> IPCGESCVWIPCISSAIGCSCKSKVCYRNG;> IPCGESCVWLPCISSAIGCSCKSKVCYRNG

Cyclotides are a large family of topologically unique peptides characterized by a head-to-tail cyclic backbone and three interlocked disulfide bonds. This combination of structural features forms a cyclic cystine knot (CCK) motif and confers cyclotides exceptional stability. Cyclotides are divided into three subfamilies: bracelet, Möbius, and trypsin inhibitor subfamilies. Since cyclotides were first reported two decades ago, studies on bracelet cyclotides have been hampered by their low synthetic yields because of poor oxidative folding efficiency.

Therefore, d-enantiomers of [I11L]cyO2 and [I11L]hD were chemically synthesized and used for quasi-racemic crystallization to determine structures of cyO2 and hyen D. The mirror-image symmetry of d-[I11L]cyO2 with l-cyO2 and d-[I11L]hD with l-hyen D was confirmed using circular dichroism (CD). The crystal structure of the quasi-racemate of wild-type cyO2 was solved in space group P1 21 1 at 1.17 Å resolution. The structure of cyO2 displays a small α-helix centered in loop 3 and a triple-strand β-sheet located in loops 4, 5, and 6. The inset of Figure 3b shows the disulfide connectivity of cyO2 is well defined by the electron density and confirms it forms the cystine knot topology, the structure of which is key to the ultrastability of cyclotides. Overall, the structure of cyO2 determined here using crystallography is similar to the solution structure previously determined by NMR spectroscopy, validating the quasi-racemic crystallography approach for structure elucidation of bracelet cyclotides. To gain more insight into the differences between bracelet and Möbius cyclotides and why they might have different folding yields, the crystal structures of cyO2 and kB1 were compared. Between the two peptides, the hydrogen bond network exhibited differences. Specifically, kB1 has more hydrogen bonds between different loops. We note, in particular, the hydrogen bond between Val-10 (loop 2) and Trp-23 (loop 5), for which an equivalent hydrogen bond to connect loop 2 to 5 is not present in cyO2.>GAMNNLVETTCKNTPNYQLCLKTLLSDKRSATGDITTLALIMVDAIKAKANQAAVTISKLRHSNPPAAWKGPLKNCAFSYKVILTASLPEA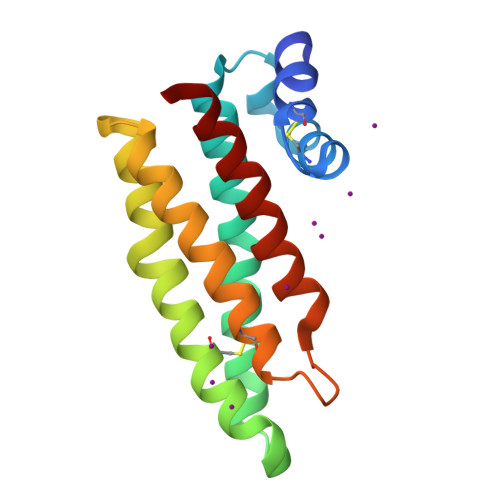IEALTKGDPKFAEDGMVGSSGDAQECEEYFKGSKSPFSALNIAVHELSDVGRAIVRNLL[2x]> MGHHHHHHQD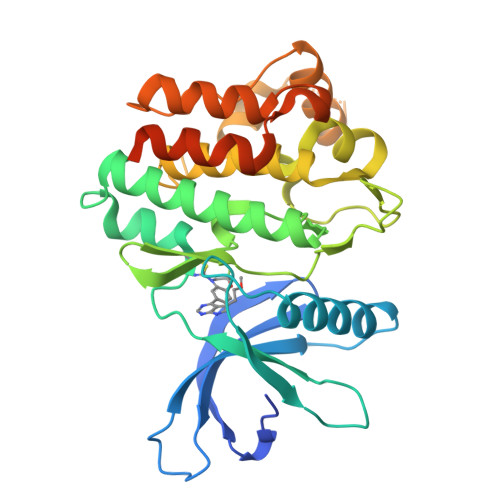PTIFEERHLKYISQLGKGNFGSVELCRYDPLGDNTGALVAVKQLQHSGPDQQRDFQREIQILKALHSDFIVKYRGVSYGPGRQSLRLVMEYLPSGCLRDFLQRHRARLDASRLLLYSSQICKGMEYLGSRRCVHRDLAARNILVESEAHVKIADFGLAKLLPLDKDYYVVREPGQSPIFWYAPESLSDNIFSRQSDVWSFGVVLYELFTYCDKSCSPSAEFLRMMGCERDVPALSRLLELLEEGQRLPAPPACPAEVHELMKLCWAPSPQDRPSFSALGPQLDMLWSGSRGCETHAFTAHPEGKHHSLSFS> SSNYCNQMMKSRNLTKDRCKPVNTFVHESLADVQAVCSQKNVACKNGQTNCYQSYSTMSITDCRETGSSKYPNCAYKTTQANKHIIVACEGN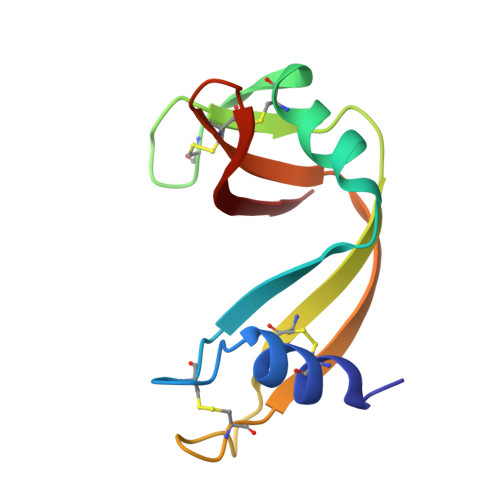PYVPVHFDASV The newly discovered CamA enzyme (named for Clostridioides difficile adenine methyltransferase A) is another orphan MTase, is present in all C. difficile genomes sequenced to date (>300), and is active in all C. difficile genomes subjected to PacBio single-molecule real-time DNA sequencing (which can detect N6-methyladenine—N6mA), but is rarely found in other bacteria. CamA-mediated methylation at CAAAAA (underlining indicates the target A) is required for normal sporulation and biofilm production by C. difficile, a key step in the disease transmission, as well as for colonization in animal models. CamA comprises an N-terminal catalytic domain (residues 1–320) and C-terminal target recognition domain (TRD; residues 320–577). The basic surface of the cleft between the two domains forms the DNA binding site with residues from both domains approaching DNA from opposite directions.

Accordingly, we purified CamA-DNA complexes and grew co-crystals, using a 13-base pair duplex containing a centrally-located A:T and with a 5′-overhang at each end (either an A or T). The complex crystallized in space group P212121, resulting in a structure determined to a resolution of 2.68 Å. In the crystallographic asymmetric unit, there are three CamA-DNA complexes (A, B and C). The CamA-bound DNA molecule undergoes major distortions at the 6-bp recognition site (labeled as 1–6), while the unrecognized flanking sequence maintains B-form. First, the bound DNA molecule is kinked between base pairs 6 and 7 (the joint between target A6 and the 3′ G7) and bent ~30°, resulting in the largest movement of ~23 Å towards one end of the DNA molecule. Third, the π-stacking force in the non-target strand is disrupted by Tyr455, which is wedged between T5–T6. Fourth, the target A6 is flipped completely out of the helix. Intriguingly, in the CamA-DNA cocrystal structure, we did not observe a bound cofactor in the SAM binding pocket next to the active-site, even though exogenous SAH was added during initial complex formation. However, the added SAH had dissociated during subsequent complex purification, probably due to the low binding affinity.

>[3x]HMDDISQDNFLLSKEYENSLDVDTKKASGIYYTPKIIVDYIVKKTLKNHDIIKNPYPRILDISCGCGNFLLEVYDILYDLFEENIYELKKKYDENYWTVDNIHRHILNYCIYGADIDEKAISILKDSLTNKKVVNDLDESDIKINLFCCDSLKKKWRYKFDYIVGNPPYIGHKKLEKKYKKFLLEKYSEVYKDKADLYFCFYKKIIDILKQGGIGSVITPRYFLESLSGKDLREYIKSNVNVQEIVDFLGANIFKNIGVSSCILTFDKKKTKETYIDVFKIKNEDICINKFETLEELLKSSKFEHFNINQRLLSDEWILVNKDDETFYNKIQEKCKYSLEDIAISFQGIITGCDKAFILSKDDVKLNLVDDKFLKCWIKSKNINKYIVDKSEYRLIYSNDIDNENTNKRILDEIIGLYKTKLENRRECKSGIRKWYELQWGREKLFFERKKIMYPYKSNENRFAIDYDNNFSSADVYSFFIKEEYLDKFSYEYLVGILNSSVYDKYFKITAKKMSKNIYDYYPNKVMKIRIFRDNNYEEIENLSKQIISILLNKSIDKGKVEKLQIKMDNLIMDSLGI> SNAMRVPYSYLERQFADIEPYLNDLREFIKTADFTLGAE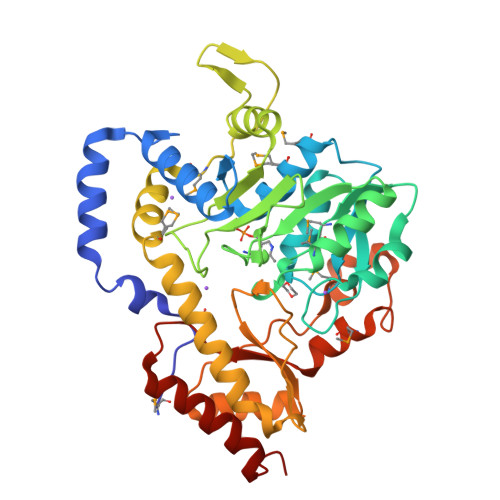LEKFEKRFAALHNAPHAIGVGTGTDALAMSFKMLNIGAGDEVITCANTFIASVGAIVQAGATPVLVDSENGYVIDPEKIEAAITDKTKAIMPVHYTGNIADMPALAKIAKKHNLHIVEDACQTILGRINDKFVGSWGQFACFSLHPLKNLNVWSDAGVIITHSDEYAEKLRLYRNHGLINRDVCVEYGINCRMDTIQAVIANRLMNQLETITEKRRGIAHLYDQSFVDLSEFIDVPVRREGVYHVFHIYVLRVKYRDQLFQYLKDNGIEVKIHYPIAMHLQPAAKSLGYQQGDFPMAEKHGEAVITLPAHPYLTEEEINYIIKKVREFYLEKHYN> GPLGSPGIPGQNTPWSSTELADAF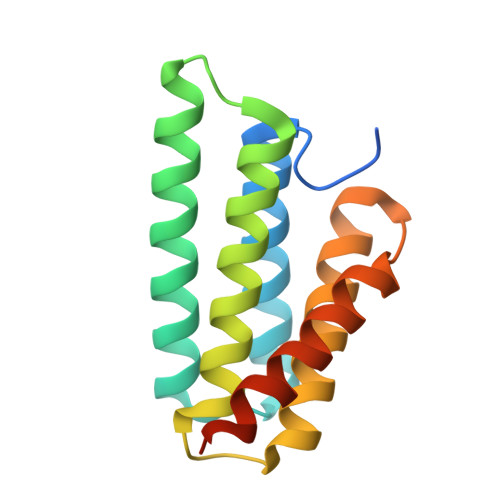INAFMNEAGRTGAFTADQLDDMSTIGDTIKTAMDKMARSNKSSKGKLQALNMAFASSMAEIAAVEQGGLSVDAKTNAIADSLNSAFYQTTGAANPQFVNEIRSLINMFAQSSANEVSYGG> 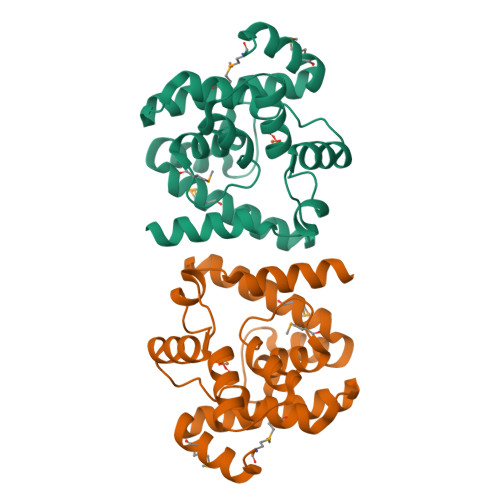GMWSYDKITDYLMNNLGEKRYKHSLGVMDTAVRLAGIYNEDTEKARIAGLVHDCAKKLPGEKIIEICTNEGYELGDEDIRNSYLLHGLAGRILAKKVIGIDDEDVLNAIEFHTTGRPNMSLLEKIIYIADYIEPGREFKGVDELRKAADEDLNKALLMSFDNTIKFVIDKGGFLHHNTIEARNYLISRKG>[2x]MAPVLGYWKIRGLAQPIRLLLEYVGDSYEEHSYGRCDGEKWQNDKHNLGLELP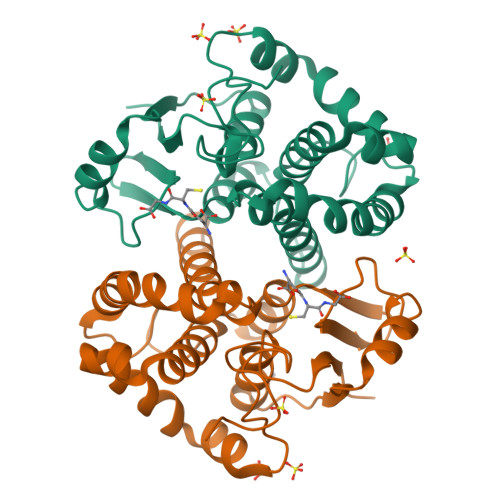NLPYYKDGNFSLTQSLAILRYIADKHNMIGNTPVERAKISMIEGGLVDLRAGVSRIAYQETFEQLKVPYLQQLPSTLRMWSQFLGNNSYLHGSTPTHLDFMFYEALDVIRYLDPTSVEAFPNLMQFIHRIEALPNIKAFMESDRFIKWPLNGWSAYFGGGDAPPK>GSMAETKAKAEDLKMQGNKAMANKDYELAINKYTEAIKVLPTNAIYYANRAAAHSSLKEYDQAVKDAESAISIDPSYFRGYSRLGFAKYAQGKPEEALEAYKKVLDIEGDNATEAMKRDYESAKKKVEQSLNL[2x];>[2x]PTVEEVD

The yeast ortholog of SGTA, Sgt2, is best understood in the context of post-translational insertion of tail-anchored (TA) proteins into the ER membrane. Sgt2 captures TA substrates after they are released from the ribosome and passes them on to the Get3 ATPase, the central targeting complex, in a process mediated by the Get4/Get5 heterodimeric scaffolding complex. Sgt2 contains an N-terminal dimerization domain, followed by the conserved, central TPR domain and a glutamine rich region toward the C-terminus. Importantly for its role, Sgt2 associates with several heat-shock proteins such as Hsp104, Hsc82 (yeast ortholog of Hsp90), and Ssa1/Ssa2 (yeast orthologs of Hsp70), which can bind directly to its central TPR domain.

Two copies of the TPR domain were present in the asymmetric unit due to non-crystallographic symmetry. All Sgt2_TPR residues could be built into electron density maps in chain A and chain B. The two peptides (chains C and D) were partially occupied and were built with care. The interaction between the Sgt2_TPR and the PTVEEVD peptide from Ssa1 is mostly driven by the formation of a two-carboxylate clamp. Most of the electrostatic interactions between the TPR domain and the peptide occur in the C-terminal EEVD region and anchor the peptide in place. In the interface between chain A and D direct backbone contacts involve hydrogen bond formation between the carboxamide sidechains of Asn141 and Asn110 in Sgt2_TPR, and the sidechain and backbone of the terminal Asp7 of the Ssa1 peptide. The guanidinium group of Arg171 forms a salt-bridge with the carbonyl main chain of Asp7 and forms an additional internal contact with Tyr169. The Arg175 sidechain interacts with the carbonyl main chain of Glu4 and Glu5 of the peptide. Phe178 and Tyr181 contribute to creating hydrophobic pockets and interact with the aliphatic part of the Pro1, Thr2, and Val3 residues. Comparing the two copies of the TPR-bound peptide indicates that, in the interface between chains B and C, the main difference is in the backbone of the N-terminal of peptide C. This is manifested through small variations in the orientation of Pro1, Thr2 and Val3 sidechains, changing hydrophobic interactions (particularly between Val3 and Phe178 of the TPR), and new electrostatic interactions between Thr2 and Asp211. It likely relates to the fact that the TPR domain helices suffer a subtle contraction to enclose the peptide in the TPR groove. The crystallographic structures we have obtained clearly show a slightly more compact conformation of the TPR where helices 1 and 7 are closer to each other in the complex structure than in the unbound TPR (See Figure S8 for a structural alignment).>NEVCYERLGCFSDDSPWAGIVERPLKILPWSPEKVNTRFLLYTNENPDNFQEIVADPSTIQSSNFNTGRKTRFIIHGFIDKGEESWLSTMCQNMFKVESVNCICVDWKSGSRTAYSQASQNVRIVGAEVAYLVGVLQSSFDYSPSNVHIIGHSLGSHAAGEAGRRTNGAVGRITGLDPAEPCFQGTPELVRLDPSDAQFVDVIHTDIAPFIPNLGFGMSQTAGHLDFFPNGGKEMPGCQKNVLSQIVDIDGIWQGTRDFAACNHLRSYKYYTDSILNPDGFAGFSCASYSDFTANKCFPCSSEGCPQMGHYADRFPGRTKGVG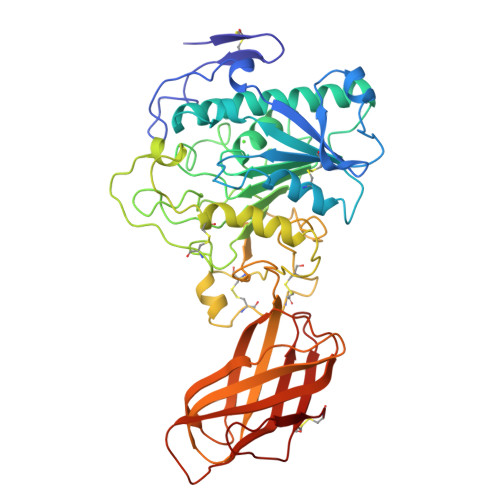QLFYLNTGDASNFARWRYRVDVTLSGKKVTGHVLVSLFGNKGNSRQYEIFQGTLKPDNTYSNEFDSDVEVGDLEKVKFIWYNNVINLTLPKVGASKITVERNDGSVFNFCSEETVREDVLLTLTAC[2x]2-AMINO-4H-1,3-BENZOXATHIIN-4-OL 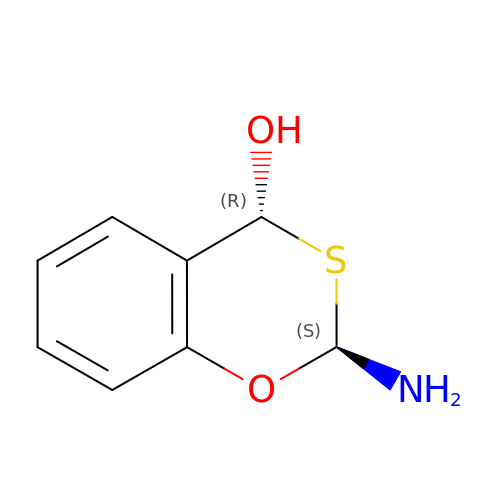| C8 H9 N O2 S | DVFUKUONLVBBEH-SFYZADRCSA-N> MGKNLSLRQDDAQHALSANTSSAYNSVYDFLRYHDRGDGLTVNGKTSYSIDQAAAQITRENVSWNGTNVFGKSANLTFKFLQSVSSIPSGDTGFVKFNAEQIEQAKLSLQSWSDVANLTFTEVTGNKSANITFGNYTRDASGNLDYGTQAYAYYPGNYQGAGSSWYNYNQSNIRNPGSEEYGRQTFTHEIGHALGLAHPGEYN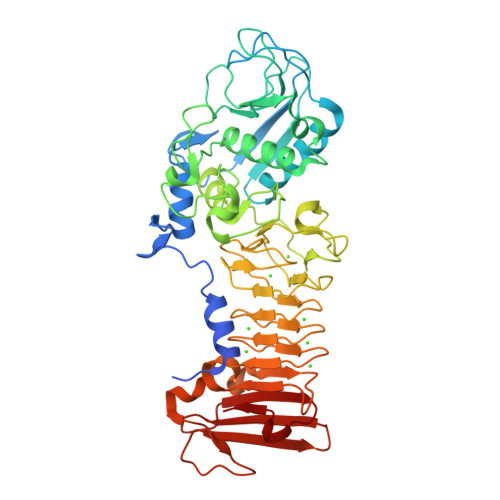AGEGDPSYNDAVYAEDSYQFSIMSFWGENETGADYNGHYGGAPMIDDIAAIQRLYGANMTTRTGDSVYGFNSNTDRDFYTATDSSKALIFSVWDAGGTDTFDFSGYSNNQRINLNEGSFSDVGGLKGNVSIAHGVTIENAIGGSGNDILVGNSADNILQGGAGNDVLYGGAGADTLYGGAGRDTFVYGSGQDSTVAAYDWIADFQKGIDKIDLSAFRNEGQLSFVQDQFTGKGQEVMLQWDAANSITNLWLHEAGHSSVDFLVRIVGQAAQSDIIV>[18x]MADVTGIALGMIETRGLVPAIEAADAMTKAAEVRLVGRQFVGGGYVTVLVRGETGAVNAAVRAGADACERVGDGLVAAHIIARVHSEVENILPKAPQA;> MKIMQVEKTLVSTNRIADMGHKPLLVVWEKPGAPRQVAVDAIGCIPGDWVLCVGS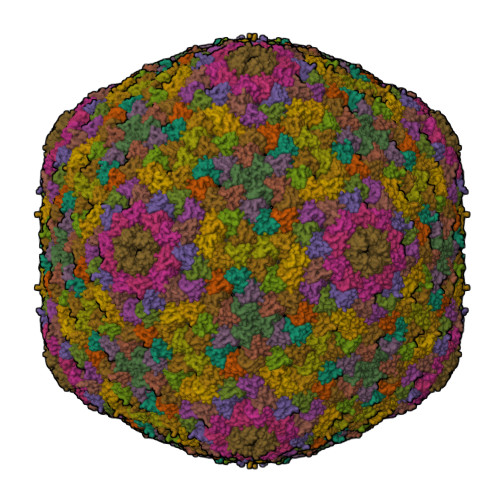SAAREAAGSKSYPSDLTIIGIIDQWNGE;>MPFCTSTPEPEAQSTEQSLTCEGQIISGTSVDASDLVTGNEIGEQQLISGDAYVGAQQTGCLPTSPRFNQTGNVQSMGFKNTNQPEQNFAPGEVMPTDFSIQTPARSAQNRITGNDIAPSGRITGPGMLATGLITGTPEFRHAARELVGSPQPMAMAMANRNKAAQAPVVQPEVVATQEKPELVCAPRSDQMDRVSGEGKERCHITGDDWSVNKHITGTAGQWASGRNPSMRGNARVVETSAFANRNVPKPEKPGSKITGSSGNDTQGSLITYSGGARG[2x]> CGAPIFQPN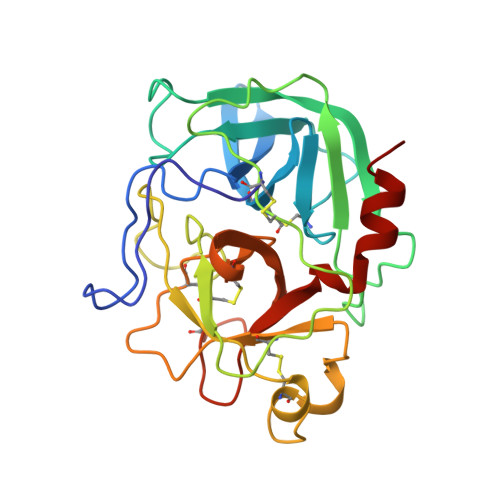LSARVVGGEDAIPHSWPWQISLQYLRDNTWRHTCGGTLITPNHVLTAAHCISNTLTYRVALGKNNLEVEDEAGSLYVGVDTIFVHEKWNSFLVRNDIALIKLAETVELGDTIQVACLPSEGSLLPQDYPCFVTGWGRLYTNGPIAAELQQGLQPVVDYATCSQRDWWGTTVKETMVCAGGDGVISACNGDSGGPLNCQADGQWDVRGIVSFGSGLSCNTFKKPTVFTRVSAYIDWINQKLQL>[4x]MNDYPPVFSKRIYKGMVAPDAVKGTPITTVYAEDADPPGMPASRVRYRVDDVQFPYPAS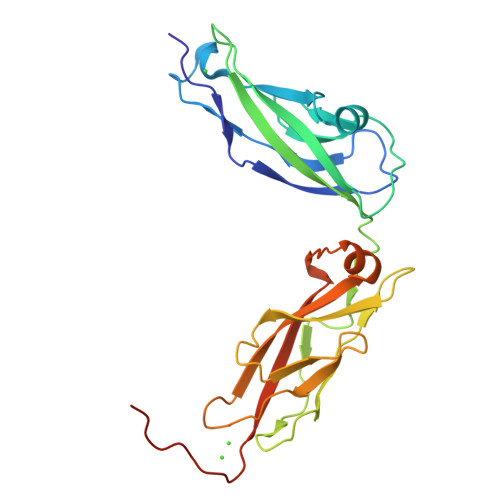IFDVEEDSGRVVTRVNLNEEPTTIFKLVVVAFDDGEPVMSSSATVRILVLHPGEIPRFTQEEYRPPPVSELAARGTVVGVISAAAINQSIVYSIVAGNEEDKFGINNVTGVIYVNSPLDYETRTSYVLRVQADSLEVVLANLRVPSKSNTAKVYIEIQDENDHPPVFLEHHHHHH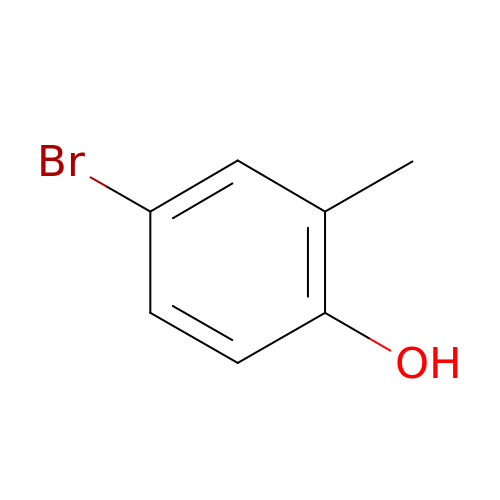4-bromo-2-methylphenol | C7 H7 Br O | IWJGMJHAIUBWKT-UHFFFAOYSA-N>[2x]SGWVWNQFFVLEEYTGTDPLYVGKLHSDMDRGDGSIKYILSGEGA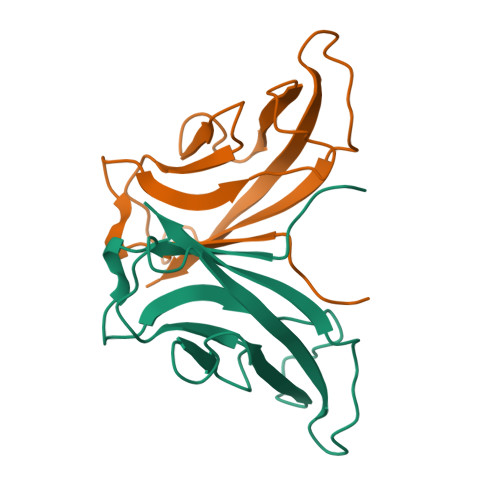GIVFTIDDTTGDIHAIQRLDREERSQYTLRAQALDRRTGRPMEPESEFIIKIQD>HHHHHHGSGPGSFLARQLGVPQPETLRRYRAGEPPLTGSLLIGGAGRVVEPLRAALEKDYDLVGNNLGGRWADSFGGL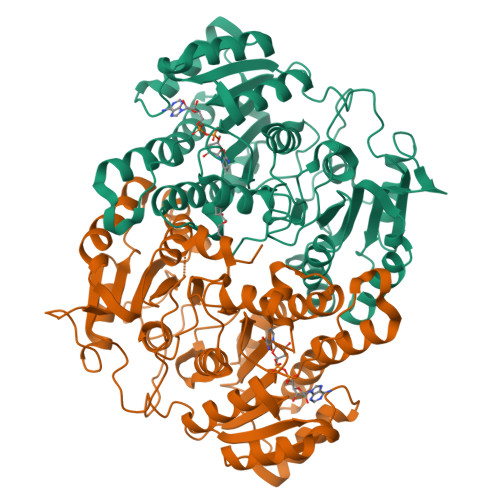VFDATGITEPAGLKGLHEFFTPVLRNLGRCGRVVVVGGTPEAAASTNERIAQRALEGFTRSLGKELRRGATTALVYLSPDAKPAATGLESTMRFLLSAKSAYVDGQVFSVGADDSTPPADWEKPLDGKVAIVTGAARGIGATIAEVFARDGAHVVAIDVESAAENLAETASKVGGTALWLDVTADDAVDKISEHLRDHHGGKADILVNNAGITRDKLLANMDDARWDAVLAVNLLAPLRLTEGLVGNGSIGEGGRVIGLSSIAGIAGNRGQTNYATTKAGMIGITQALAPGLAAKGITINAVAPGFIETQMTAAIPLATREVGRRLNSLLQGGQPVDVAEAIAYFASPASNAVTGNVIRVCGQAMIGA[4x]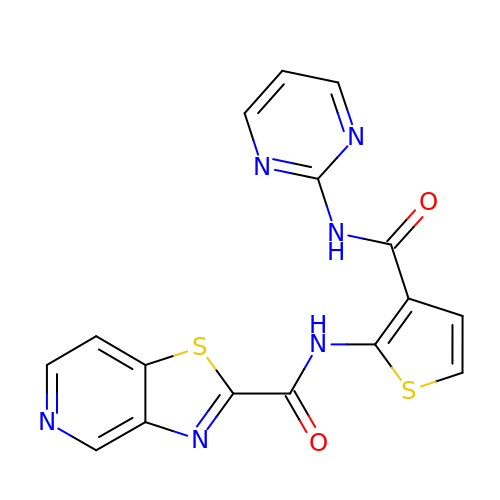~{N}-[3-(pyrimidin-2-ylcarbamoyl)thiophen-2-yl]-[1,3]thiazolo[4,5-c]pyridine-2-carboxamide | C16 H10 N6 O2 S2 | AJCHWWGZVVPQDY-UHFFFAOYSA-N>[4x]EAYTLSTLAALPAAEIVRLANSQSSSGLPLPKADPATVKATDDFIDSLQGKAAHDQKQKLGDQ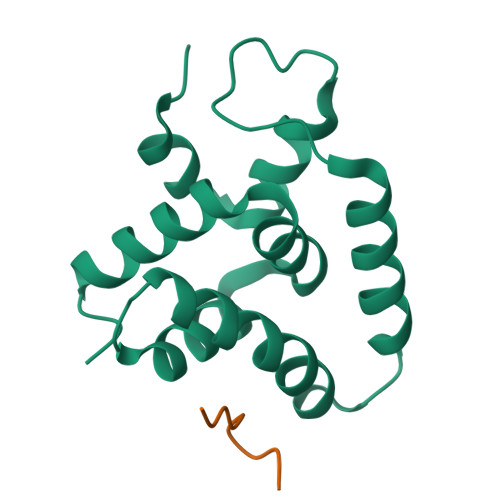LFKKIRTFGVKGAPKLTIHLLDSEDLRALAHLMNSYEDVLKEKVQHKVAAGLNKFGVKGAPKLTIHLLDSED;>KLKPYVFDY[4x]(3S)-3-AMINO-1-(CYCLOPROPYLAMINO)HEPTANE-2,2-DIOL 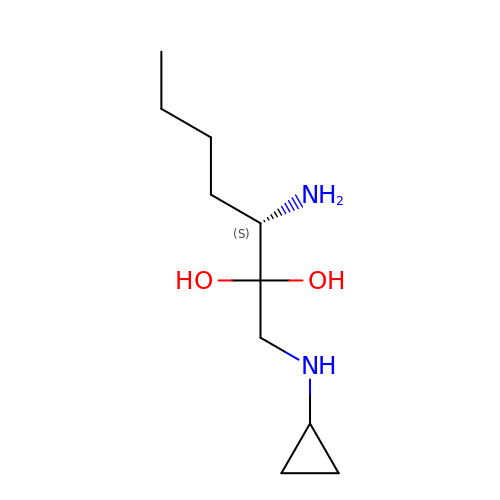| C10 H22 N2 O2 | AYBDGNNJGBFOBQ-VIFPVBQESA-N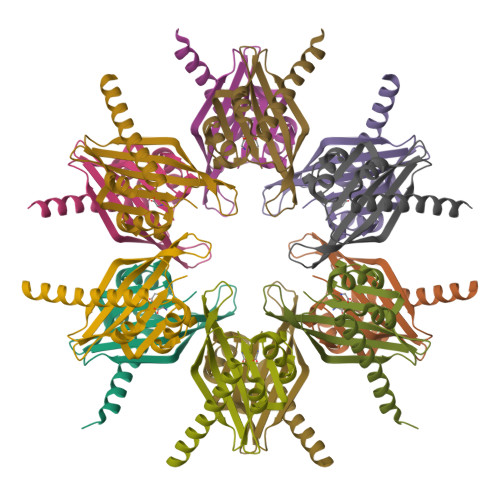>[6x]SMTEDEDLKVRKQEIIKITEQLIEAINNGDFEAYTKICDPGLTSFEPEALGNLVEGMDFHKFYFENLLSKNSKPIHTTILNPHVHVIGEDAACIAYIRLTQYIDGQGRPRTSQSEETRVWHRRDGKWLNVHYHCSGAPAAPRQ>MREHIGSQEPVILIDKIERCLVVEWYENNIRREQRISYKKYGNDKAKLRAKELIEKLKSGITFEQLYPDKGPPIVRVFENVGVYNVSL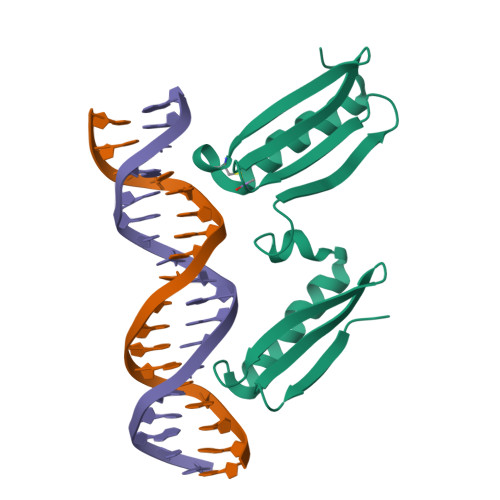IRDRIEREWRVEWLENGVPMKARWSCKKVGNDEAQKRADTFAQSMIKGIFN[3x]Here we report the crystal structures of a novel transcriptional repressor RolR and its complex with the regulator resorcinol. The RolR protomer is folded as two domains, the DNA-binding domain at N-terminal and the signal-receiving domain at C-terminal. In addition, RolR is the sole TetR-type regulator that has been identified for regulation of aromatic catabolism. RolR is an all-helix protein and each subunit is composed of 9 α helices (h1, h2, h4–h10) and two 310 helices for h3 and g1, a stretch between h1 and h2.

The crystal structure of the apo-RolR is solved by the molecular replacement method using the N- and C-domains of res-RolR structure as initial models. The structure is refined to 3.6 Å resolution and the statistics are listed in Table 1. At this resolution, the electron density maps are qualified for fitting well to all mainchains and about 1/3 sidechains, which make the reliability to analysis the apo-RolR structure on the mainchain and secondary structure level with some sidechains for a part of residues. The final apo-RolR model contains two dimers, AB and CD, in the asymmetric unit, which have the dimeric organization same as that in res-RolR. The general structures of these two dimers are very similar with a Cα r.m.s.d of 0.9 Å, we therefore use the dimer CD in the following comparative analysis due to its better fitting to density maps. The apo-RolR structure shows the similar general fold to that of res-RolR, but the DNA binding domain shows some relative movement in comparison with that in complex res-RolR (2a, 2c). Besides, some subtle distinctions for h3 and g1, the stretch between h1 and h2, are observed, which take a short 310 helix and a loop, respectively. Structural comparison shows that the frameworks of the binding pockets in apo- and res-RolR structures are very similar without obvious conformational change at mainchains. The structural comparison between apo-RolR and res-RolR show that the orientations of DNA-binding motif h2–h3 and h2′–h3′in dimerization have been swung about 10 degree referring to the C-domain from the ligand-free form to the ligand-binding form, which further make the center-to-center separation of the DNA-binding domain (defined as the distance between residues Tyr68 in h3 and h3′) shortened from 34.9 Å to 30.1 Å upon the ligand-binding. In this way, residues Arg122 and Arg74 restrain the conformations of residues Glu45, Arg46, Val48 and Val51 via hydrogen bonds in the ligand-bound form but not in the ligand-free form after the 10 degree swing.

>[4x]HHHHHHSSGLVPRGSHMPTPSQHKDASTAQTDNQVPTGRRAQKREQTRARLITSARTLMAERGVDNVGIAEITEGANIGTGTFYNYFPDREQLLQAVAEDAFESVGIALDQVLTKLDDPAEVFAGSLRHLVRHSLEDRIWGGFFIQMGAAHPVLMRILGPRARRDLLHGLETGRFTIEDLDLATTCTFGSLIAAIQMALSADQDSNDDKDQIFAAAMLRMVGVQAAEAREIASRPLPEISPVKPQ>[2x]MILIRGLTRVITFDDQERELEDADILIDGPKIVAVGKDLSDRSVSRTIDGRGMIALPGLINSHQHLYEGAMRAIPQLERVTMASWLEGVLTRSAGWWRDGKFGPDVIREVARAVLLESLLGGITTVADQHLFFPGATADSYIDATIEAATDLGIRFHAARSSMTLGKSEGGFCDDLFVEPVDRVVQHCLGLIDQYHEPEPFGMVRIALGPCGVPYD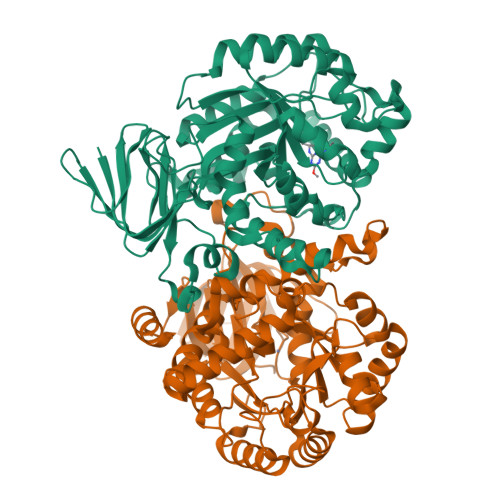KPELFEAFAQMAADYDVRLHTHFYQPLDAGMSDHLYGMTPWRFLEKHGWASDRVWLAHAVVPPREEIPEFADAGVAIAHLIAPDLRMGWGLAPIREYLDAGITVGFGTTGSASNDGGNLLGDLRLAALAHRPADPNEPEKWLSARELLRMATRGSAECLGRPDLGVLEEGRAADIACWRLDGVDRVGVHDPAIGLIMTGLSDRASLVVVNGQVLVENERPVLADLERIVANTTALIPKNL> MTSIRAVVFDAYGTLFDVYSVAARAEQLFPGKGEALSVLWRDR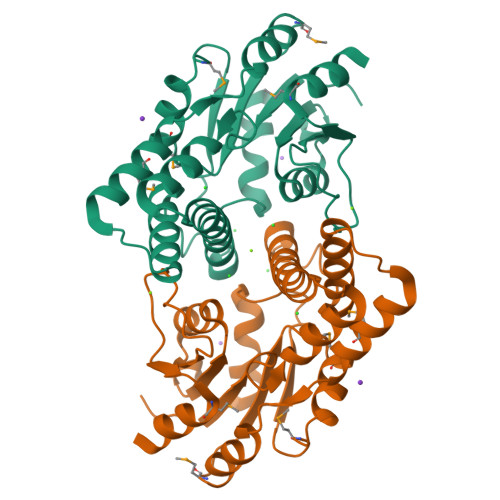QIDYTRIRSLAGPSGEHYKPFWDVTVDALRYACARLNLPLGNHAEATLMREYACLSAFPENVPVLRQLREMGLPLGILSNGNPQMLEIAVKSAGMSGLFDHVLSVDAVRLYKTAPAAYALAPRAFGVPAAQILFVSSNGWDACGATWHGFTTFWINRLGHPPEALDVAPAAAGHDMRDLLQFVQARQSMR5'-O-[N-(3-Indolepropionic 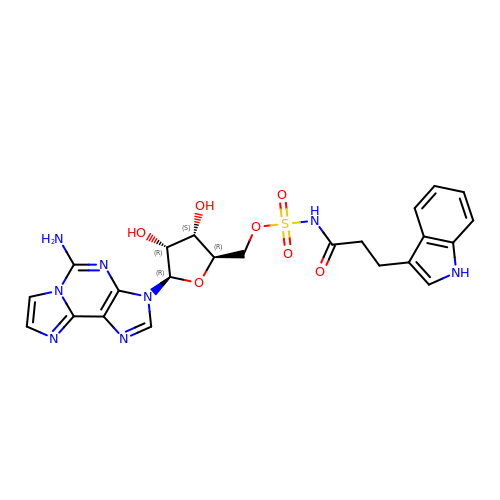acid)sulfamoyl] 2-aminoethenoadenosine | C23 H24 N8 O7 S | UXQPTDCOLAEKOF-CIVUBGFFSA-N N-methyl-N-[2-oxo-2-(piperidin-1-yl)ethyl]methanesulfonamide 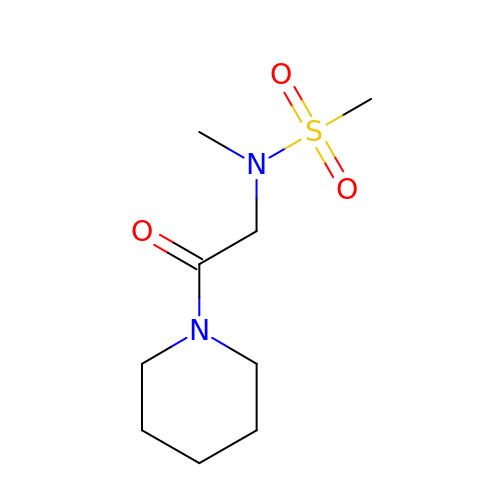| C9 H18 N2 O3 S | CPSZUJVUZDHXHY-UHFFFAOYSA-N> MSAIKPD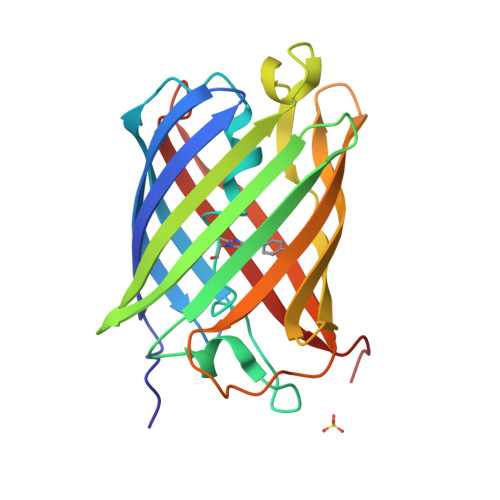MKIKLRMEGNVNGHHFVIDGDGTGKPFEGKQSMDLEVKEGGPLPFAFDILTTAFXNRVFAKYPDNIQDYFKQSFPKGYSWERSLTFEDGGICNARNDITMEGDTFYNKVRFYGTNFPANGPVMQKKTLKWEPSTEKMYVRDGVLTGDVETALLLEGNAHYRCDFRTTYKAKEKGVKLPGAHFVDHCIEILSHDKDYNKVKLYEHAVAHSGLPN> GSMFPHHSITESVNYDVKTFGSSLPVKVMEALTLAEVDDQLTINIDEGGWACLVCKEKLIIWKIALSPITKLSVCKELQLPPSDFHWSADLVALSYSSPSGEAHSTQAVAVMVATREGSIRYWPSLAGEDTYTEAFVDSGGDKTYSFLTAVQ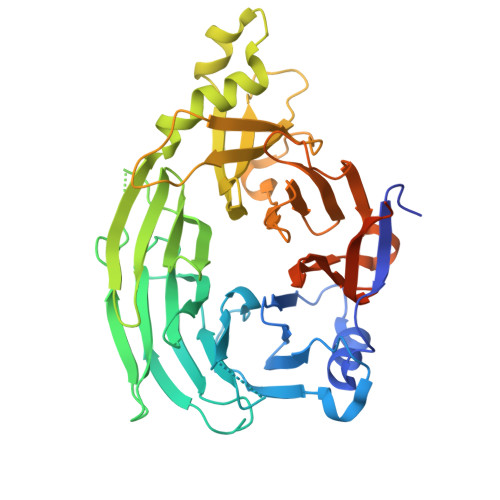GGSFILSSSGSQLIRLIPESSGKIHQHILPQGQGMLSGIGRKVSSLFGILSPSSDLTLSSVLWDRERSSFYSLTSSNISKWELDDSSEKHAYSWDINRALKENITDAIWGSESNYEAIKEGVNIRYLDLKQNCDGLVILAAAWHSADNPCLIYYSLITIEDNGCQMSDAVTVEVTQYNPPFQSEDLILCQLTVPNFSNQTAYLYNESAVYVCSTGTGKFSLPQEKIVFNAQGDSVLGAGACGGVPIIFSRNSGLVSITSRENVSILAEDLEGSLASSVAGPNSESMIFETTTKNETIA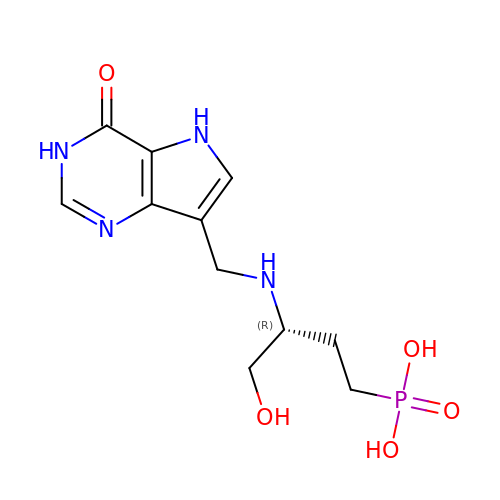[(3R)-4-hydroxy-3-{[(4-oxo-4,5-dihydro-3H-pyrrolo[3,2-d]pyrimidin-7-yl)methyl]amino}butyl]phosphonic acid | C11 H17 N4 O5 P | YYXVNWBGVIIBOW-MRVPVSSYSA-N> GPDSMRFKPGVI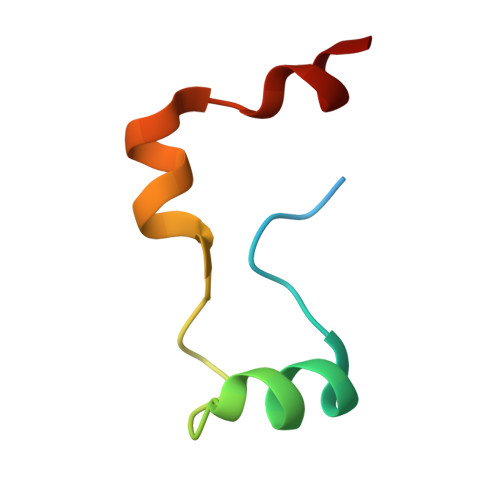SEELQDALGVTDKSLPPFIYRMRQLGYPPGWLK> MPKPINVRVTTMDAELEFAIQPNTTGKQLFDQVVKTVGLREVWFFGLQYVDSKGYSTWLKLNKKVTQQDVKKENPLQFKFRAKFFPEDVSEELIQEITQRLFFLQVKEAILNDEIYCPPETAVLLASYAVQAKYGDYNKEIHKPGYLANDRLLPQRVLEQHKLTKEQWEERIQNWHEEHRGMLR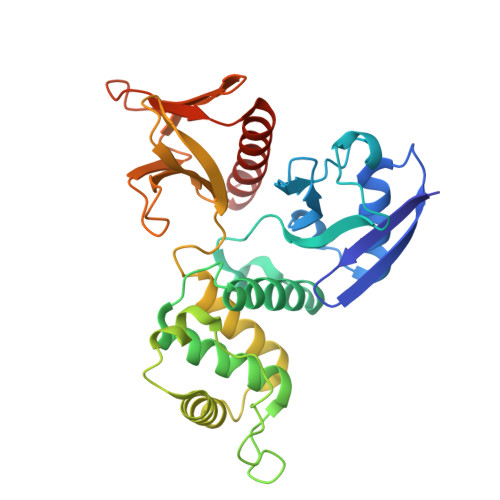EDSMMEYLKIAQDLEMYGVNYFEIKNKKGTELWLGVDALGLNIYEHDDKLTPKIGFPWSEIRNISFNDKKFVIKPIDKKAPDFVFYAPRLRINKRILALCMGNHELYMRRRK>[4x]MAHGPFNAQGFTDFDSLSGTSTTWVNELGSVMTIDVDRKGGVTGYFV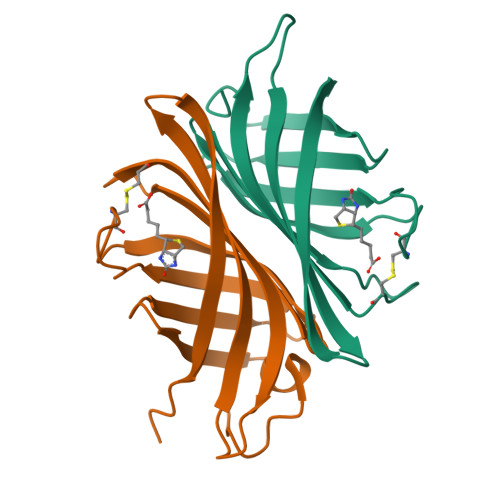NNAPGTGCRGLPYDLSGHAHGSTIAFSVVWSNGIADCRSATSWAGYARKTFGGGVQIVTQWSLAFVGKAGGKIETGQNVFTYQAYDAQPSPADK> LESPGFMVHKKLK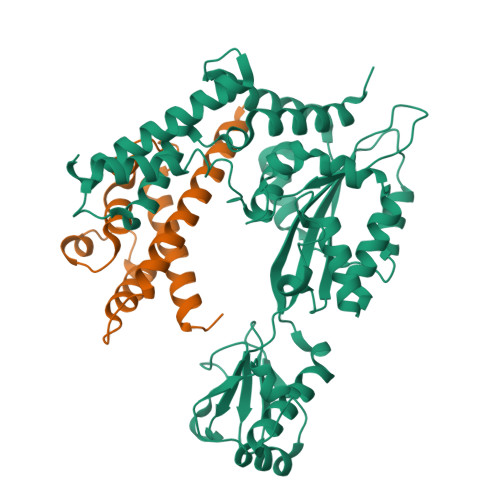SMSQSYGVMMTGVPAEVLGQMQAERSIPSINKTGNLKQQIAKEVSKVCHMMTEPTQSAGQASNDVCELLLGKIEAEKFHFTKYEALSADGDNLKNVLENTAPSSTNLLIRFEIDREDPPIVLVKTKNENFNPETAVKNKIYLLENKLYFIDKMGNLFNLGPGKKKCTQLFNAIGDSAEYSLCDPFVLEEPEKPEDFAISEIVDIFNEQKERFDFWIGSHSFTIYIPQTLGESPRQFYPYQAYFGSHTLQDWFVSDKDEYLSRIGIDKYIEKLAVLGKTTNTKERSDIYAEFFSKRGREAFFCAHLNEKRQPLRVKFKITEINPELALKNLQETQEFIDTHPGENPSDKVENYRNRAKLAMTEHLESLLDI;> HMFFKDYQKKNVMRLLQDSLEKIINEWLKTDDESHTKLKSLQELSEMDINATSFAEHSPLPDFVTRLWLDPHKALDAMDKNISKNEIRKLIKETAREIELVFTHQK methyl 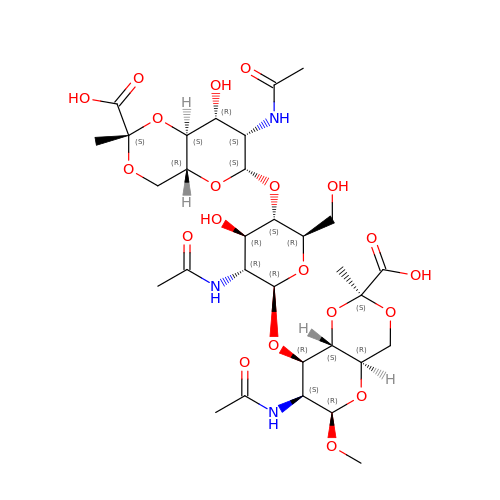2-acetamido-4,6-O-[(1S)-1-carboxyethylidene]-2-deoxy-beta-D-mannopyranosyl-(1->4)-2-acetamido-2-deoxy-beta-D-glucopyranosyl-(1->3)-2-acetamido-4,6-O-[(1S)-1-carboxyethylidene]-2-deoxy-beta-D-mannopyranoside | C31 H47 N3 O20 | TVHSRPKDDVTCLX-FLRWZPIQSA-N>[4x]EGEDLTLEEKAEICSELELQQKYVDIASNIIGDLSSLPIAGKIAGTIAAAAMTATHVASGRLDIEQTLLGCSDLPFDQIKEVLENRFNEIDRKLDSHSAALEEITKLVEKSISVVEKTRKQMNKRFDEVMKSIQDAKVSPIISKINNFARYFDTEKERIRGLKLNDYILKLEEPNGILLHFKESRTPTDDSLQAPLFSIIEEGYAVPKSIDDELAFKVLYALLYGTQTYVSVMFFLLEQYSFLANHYYEKGYLEKYDEYFNSLNNVFLDFKSSLVGTGTSNNEGLLDRVLQVLMTVKNSEFLGLEKNGVDEMLNEKINLFNKIKEEIEGKQKMTLSETPENFAQISFDKDITTPIGDWRDGREVRYAVQYASETLFSKISHWSDPVSVREKACPTLRMPVDQTRRNVLVFRKFDSSKPQLVGEITPYLSNFIDIDRDLYNAASNPDSAVGFKEFTKLNYDGANIRATFDHGRTVFHAAAKSGNDKIMFGLTFLAKSTE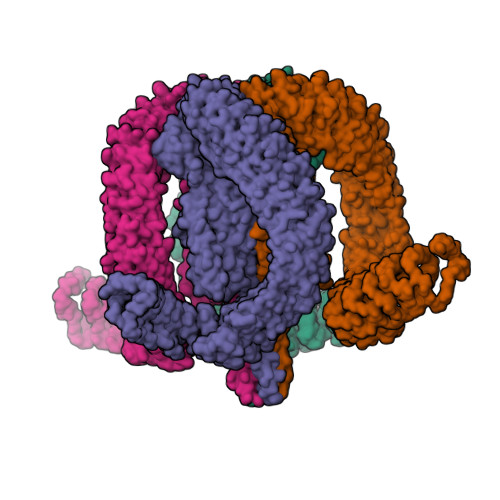LNQPDKKGYTPIHVAADSGNAGIVNLLIQRGVSINSKTYHFLQTPLHLAAQRGFVTTFQRLMESPEININERDKDGFTPLHYAIRGGERILEAFLNQISIDVNAKSNTGLTPFHLAIIKNDWPVASTLLGSKKVDINAVDENNITALHYAAILGYLETTKQLINLKEINANVVSSPGLLSALHYAILYKHDDVASFLMRSSNVNVNLKALGGITPLHLAVIQGRKQILSLMFDIGVNIEQKTDEKYTPLHLAAMSKYPELIQILLDQGSNFEAKTNSGATPLHLATFKGKSQAALILLNNEVNWRDTDENGQMPIHGAAMTGLLDVAQAIISIDATVVDIEDKNSDTPLNLAAQNSHIDVIKYFIDQGADINTRNKKGLAPLLAFSKKGNLDMVKYLFDKNANVYIADNDGMNFFYYAVQNGHLNIVKYAMSEKDKFEWSNTDNNRRDECPNEECAISHFAVCDAVQFDRIEIVKYFVGTLGNFAICGPLHQAARYGHLDIVKYLVEEEFLSVDGSKTDTPLCYASENGHFTVVQYLVSNGAKVNHDCGNGMTAIDKAITKNHLQVVQFLAANGVDFRRKNSRGTTPFLTAVAENALHIAEYLIREKRQDININEQNVDKDTALHLAVYYKNLQMIKLLIKYGIDVTIRNAYDKTALDIAIDAKFSNIVEYLKTKSG> MNLKLQLKILSFLQFCLWGSWLTTLGSYMFVTLKFDGASIGAVYSSLGIAAVFMPALLGIVADKWLSAKWVYAICHTIGAITLFMAAQVTTPEAMFLVILINSFAYMPTLGLINTISYYRLQNAGMDIVTDFPPIRIWGTIGFIMAMWVVSLSGFELSHMQLYIGAALSAILVLFTLTLPHIPVAKQQANQSWTTLLGLDAFALFKNKRMAIFFIFSMLLGAELQITNMFGNTFLHSFDKDPMFASSFIVQHASIIMSISQISETLFILTIPFFLSRYGI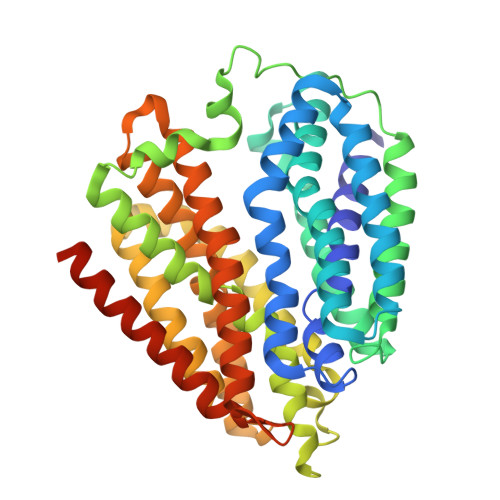KNVMMISIVAWILRFALFAYGDPTPFGTVLLVLSMIVYGCAFAFFNISGSVFVEKEVSPAIRASAQGMFLMMTNGFGCILGGIVSGKVVEMYTQNGITDWQTVWLIFAGYSVVLAFAFMAMFKYKHVRVPTGTQTVSH> EREALPPQKIEVLVLLPQDDSYLFSLTRVRPAIEYALRSVEGNGTGRRLLPPGTRFQVAYEDSDCGNRAL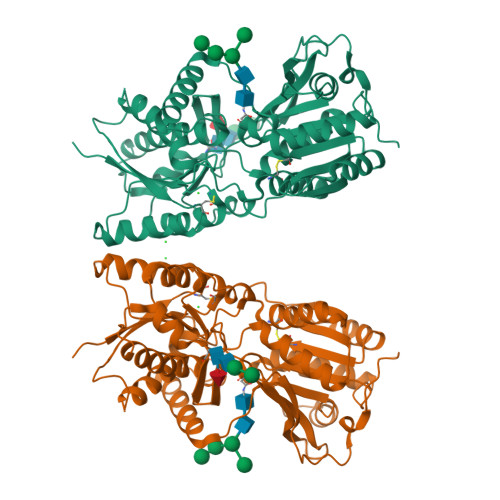FSLVDRVAAARGAKPDLILGPVCEYAAAPVARLASHWDLPMLSAGALAAGFQHKDSEYSHLTRVAPAYAKMGEMMLALFRHHHWSRAALVYSDDKLERNCYFTLEGVHEVFQEEGLHTSIYSFDETKDLDLEDIVRNIQASERVVIMCASSDTIRSIMLVAHRHGMTSGDYAFFNIELFNSSSYGDGSWKRGDKHDFEAKQAYSSLQTVTLLRTVKPEFEKFSMEVKSSVEKQGLNMEDYVNMFVEGFHDAILLYVLALHEVLRAGYSKKDGGKIIQQTWNRTFEGIAGQVSIDANGDRYGDFSVIAMTDVEAGTQEVIGDYFGKEGRFEMRPNVKYPWGPLKLRIDENRIVEHTNSSPCKSCGLEESAVT> MGCVAETGDCGLPPDVPNAQPALEGRTSFPEDTVITYKCEESFVKIPGEKDSVICLKGSQWSDIEEFCNRSCEVPTRLNSASLKQPYITQNYFPVGTVVEYECRPGYRREPSLSPKLTCLQNLKWSTAVEFCKKKSCPNPGEIRNGQIDVPGGILFGATISFSCNTGYKLFGSTSSFCLISGSSVQWSDPLPECREIYCPAPPQIDNGIIQGERDHYGYRQSVTYACNKGF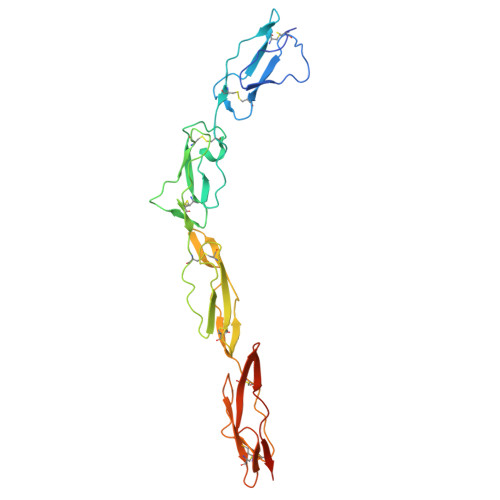TMIGEHSIYCTVNNDEGEWSGPPPECRGGTKHHHHHH ETHYL 4-[(2-CYANOETHYL)SULFANYL]-6-{[6-(PIPERAZIN-1-YL) | C25 H27 N5 O3 S | 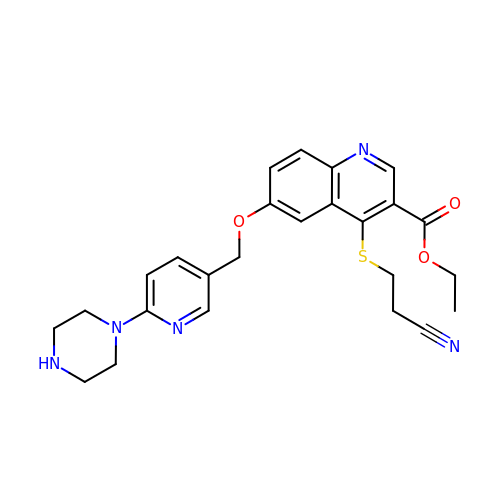BOXNSEIJTUHQDY-UHFFFAOYSA-N> MANIVNFTDKQFENRLNDNLEELIQGKKAVESPTAFLLGGQPGSGKTSLRSAIFEETQGNVIVIDNDTFKQQHPNFDELVKLYEKDVVKHVTPYSNRMTEAIISRLSDQGYNLVIEGTGRTTDVPIQTATMLQAKGYETKMYVMAVPKINSYLGTIERYETMYADDPMTARATPKQAHDIVVKNLPTNLETLHKTGLFSDIRLYNREGVKLYSSLETPSISPKETLEKELNRKVSGKEIQPTLERIEQKMVLNKHQETPEFKAIQQKLESLQPPT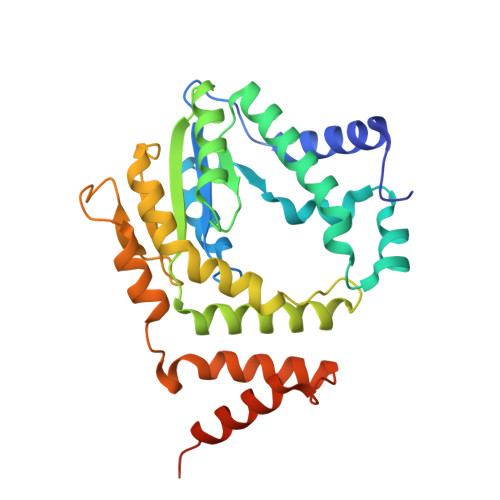PPIPKTPKLPGI For rotaviruses (RVs), which are the major causative agents of life-threatening gastroenteritis in children under the age of 5 years and result in 453,000 deaths worldwide annually, recognition of specific cellular glycans for initial cell attachment is mediated by the distally located VP8* domain of the spike protein VP4. Although structurally conserved with a galectin-like fold, sequence-wise VP8* is the least conserved among RV structural proteins contributing to a phylogeny consisting of 37 [P] genotypes9. Our crystallographic analyses provide the structural basis to explain the unique glycan specificity exhibited by a neonate-specific bovine-human reassortant RV strain and its parental bovine strain, each belonging to the P genotype. We have shown that P VP8* exhibits a novel glycan-binding site that adapts to a differential recognition of precursor glycans, which are the core elements of HBGA and human/bovine milk glycans.

To understand how the genotypic sequence variations alter the structure and influence the glycan specificity in the neonate-specific P HRV, we determined the crystal structure of VP8* of a P human neonatal RV strain N155 isolated from a neonate with severe gastrointestinal disease in India28. As in other VP8* structures, the P HRV VP8* adopts a galectin-like fold with two twisted antiparallel β-sheets consisting of strands A, L, C, D, G, H and M, B, I, J, K, respectively. The two β-sheets are separated by a distinct cleft, which constitutes the glycan-binding site in the VP8* of ARVs and P HRV. This cleft is noticeably wider in the P HRV VP8* than that in the ARV VP8* structures or the P VP8*; however, the width is similar to that observed in the VP8* of the globally dominant P and P HRVs. Consistent with its distinct glycan-binding profile, the structure-based sequence alignment of representative VP8*s shows that the residues at the known Sia or A-HBGA-binding site are altered significantly in P HRV N155. For instance, R101 in the VP8*s of ARV and P HRV, which is critical for glycan binding, is altered to a phenylalanine, whereas the conserved Y188 and Y189 are replaced by glycine and threonine, respectively, in the P HRV VP8*. In addition to these amino acid changes, which may impact glycan specificity, there are significant structural alterations in the P HRV VP8* structure, particularly in the I-J and J-K loops, which may also influence glycan specificity. A distinguishing feature of the P VP8* is that glycan binding occurs in a previously uncharacterized binding pocket and the binding cleft is noticeably wider. Based on the currently available VP8* structures, a structure-based analysis of the VP8* sequences indicates that the wider cleft strongly correlates with a deletion at position 135, and a significant change at position 101, which is a conserved arginine residue contributing to glycan interactions in the VP8*s with a narrow cleft27.

>[2x]GSALDGPYTPDSSNLPSNYWYLINPLNDGVVFSVTNNSTFWMFTYLILPNTAQTNVTVNVMNETVNISIDNSGSTYRFVDYFKTSSTQSYRQRNYLITEHRLQAYRRDESGNISNYWGSSTYGDLRVGTYFNPVLNAVINLNADFYIIPDSQQEKCTEYIKGGL> MVSKGE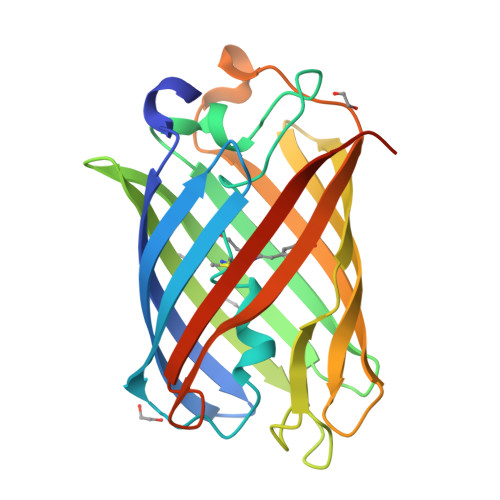ELIKEEMPMKVVLEGTVNGHQFKCTGEGEGRPYEGVQTMRIKVIEGGPLPFAFDILATSFMYGSRTFVKHPKGIPDYFKQSFPEGFTWERVTRYEDGGVVTVTQDTSLQDGVLIYNAKVRGVNFPSNGPVMQKKTKGWEPNTEMIYPADGGLRGYTDMALKVDGGGHLHCSFVTEYRSKKTVGNIKMPGVYAIDHRLERIEESDNETYVVQREVAVAKYSNLGGGMDELYK> GTEGSWLFSTCGASGRHGPTQTQCDGAYAGTSVVVTVGAAGQLRGVQLWRVPGPGQYLISAYGAAGGKGAKNHLSRAHGVFVSAIFSLGLGESLYILVGQQGEDACPGGSPESQLVCLGESRAVEEHAAMDGSEGVPGSRRWAGGGGGGGGATYVFRVRAGELEPLLVAAGGGGRAYLRPRDRGRTQASPEKLENRSEAPGSGGRGGAAGGGGGWTSRAPSPQAGRSLQEGAEGGQGCSEAWATLGWAAAGGFGGGGGACTAGGGGG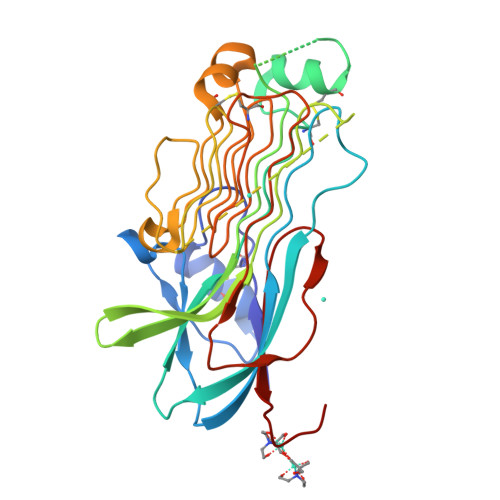GYRGGDASETDNLWADGEDGVSFIHPSSELFLQPLAVTENHGEVEIRRHGTDEVD> MDEEIFDNPIQKLNYNIRTEESGSLLKYLQSQKSNFTDSKKFISFKQKGNDSVGIRKEITQKKSFPLDNGFIGTVADPFIAIAFQISDRFNIDEYLACRILYSVVDHSTTRDEKELIELSEKFIYQNRSCYLQFLREILHTLQSRDSVNDINHSKMKHDILQSFIGELISEQTNDKNIVTILIKTLEEKVKDMNGTVNPLECCFRVKECIQIVECLFLISIQFTIKEDIIKLYIRVLNQVIEKEKREDSILKKSLFEIMFTLYFTIFAVF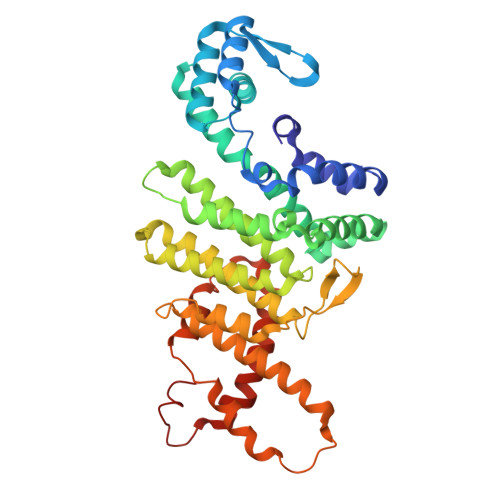DNVKNSQVFNAIEKRYTFNEISSTDSIENEIKQIDNQHPIKSSLYAIFNIILIAKENNNSNSNSNSNSNSNSNSNNNNNRITPENDSYKFLLQAVQTQEYQLSPLNILFGSFINILSCRFLSNLSSHPTKKDILY2-[(3-HYDROXY-2-METHYL-5-PHOSPHONOOXYMETHYL-PYRIDIN-4-YLMETHYL)-AMINO]-PROPIONIC 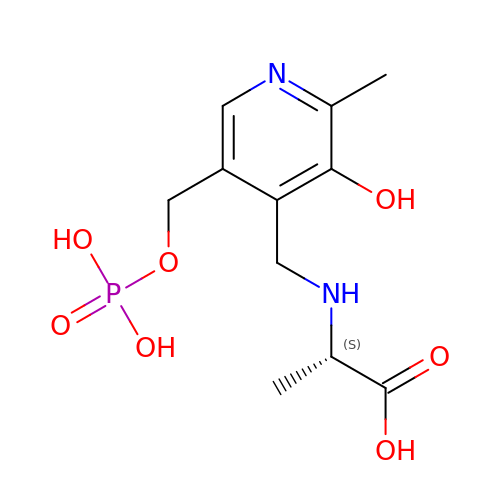ACID | C11 H17 N2 O7 P | WACJCHFWJNNBPR-ZETCQYMHSA-N>MNIISTSVYVGPNVYASIPLIRLVIDLNPHYITQLASMGSEVLENLEKVIPTLKTEQDAKLQHKLEELRQAPQQQIGELVAILALHLQRLAGQKGGAAFSAYCHEDETEILYSYESEEIGIEAGEVVCDMLVALAKAHEAGDQIDLNRDVKGFLRYADRFALGPSALALVQAAEERNIPWYRLNDASLIQVGQGKYQKRIEAALTSGTSHIAVEIAGDKNVCNQLLQDLGLPVPKQRVVYDIDDAVRAARRVGFPVVLKPLDGNHGRGVSVNLTTDEAVEAAFDIAMSEGSAVIVESMLYGDDHRLLVVNGELVAAARRVPGHIVGDGKHNVEALIEIVNQDPRRGVGHENMLTKIELDEQALKLLAEKGYDKDSIPAKDEVVYLRRTANISTGGTAIDVTDTIHPENKLMAERAIRAVGLDIGAVDFLTTDITKSYRDIGGGICEVNAGPGLRMHISPSEGPSRDVGGKIMDMLFPQGSQSRVPIAAITGTNGKTTCSRMLAHILKMAGHVVGQTSTDAVYIDGNVTVKGDMTGPVSAKMVLRDPSVDIAVLETARGGIVRSGLGYQFCDVGAVLNVSSDHLGLGGVDTLDGLAEVKRVIAEVTKDTVVLNADNAYTLKMAGHSPAKHIMYVTRDAENKLVREHIRLGKRAVVLEKGLNGDQIVIYENGTQIPLIWTHLIPATLEGKAIHNVENAMFAAGMAYALGKNLDQIRIGLRTFDNTFFQSPGRMNVFDKHGFRVILDYGHNEAAVGAMTELVDRLNPRGRRLLGVTCPGDRRDEDVVAI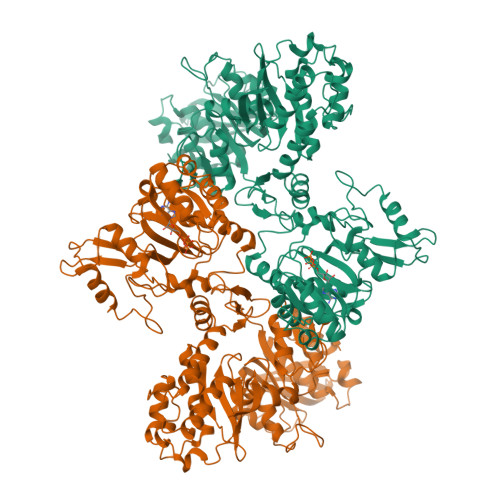AAKVAGHFDEYYCHRDDDLRGRAPDETPKIMRDALIQLGVPESRIHIVEQEEDSLAAVLTEAQVDDLVLFFCENITRSWKQIVHFTPEFNIENDHETLELKIAEQGFDIPEGYHAVSNDRGVMILPRGENLYFQGHHHHHHHH[2x]Our enzyme of interest is isocyanide hydratase (ICH), which catalyzes the irreversible hydration of isocyanides to N-formamides via formation of a cysteine-derived thioimidate intermediate. ICHs are commonly found in pseudomonad bacteria and soil-dwelling fungi and likely serve a defensive role against isocyanide natural products produced by competing microbes. Asp17 is catalytically essential in ICH, where it is proposed to act as a general acid/base. In addition to its intrinsic biochemical interest, ICH is a useful model system for catalysis-activated enzyme dynamics.

By contrast, G150T ICH samples this conformational ensemble at rest because of steric effects of the G→T substitution at residue 150. Because G150T stably adopts a state that is transiently populated by the wild-type enzyme, it is a useful tool for studying how ICH conformational ensembles change during the catalytic cycle. The movement of atoms along “softer” internal degrees of freedom in the enzyme is further supported by comparison of a cryogenic (100 K) structure with the 274 K synchrotron and 298 K XFEL structures of G150T ICH. The cryogenic structure superimposes on the XFEL structure of G150T with all-atom RMSD of 0.45 Å (Cα RMSD = 0.21 Å), and many Fo(synchrotron)-Fo(XFEL) map peaks lie in the direction of displacements between the cryogenic and XFEL structures. Despite having nearly identical overall structures, isomorphous difference (Fo-Fo) electron density maps calculated between the 274 K synchrotron and 298 K XFEL datasets for G150T ICH showed features that aligned with principal axes of anisotropic ADPs and with minor shifts in atomic position between these higher temperature structures and a cryogenic (100 K) structure.

>[2x]GSHMAVQIGFLLFPEVQQLDLTGPHDVLASLPDVQVHLIWKEPGPVVASSGLVLQATTSFADCPPLDVICIPGGTGVGALMEDPQALAFIRQQAARARYVTSVCTGSLVLGAAGLLQGKRATTHWAYHELLAPLGAIPVHERVVRDGNLLTGTGITAGIDFALTLAAELFDAATAQRVQLQLEYAPAPPFNAGSPDTAPASVVQQARQRAADSLHKRREITLRAAARLAAG>[4x]MVSKGEEDNMASLPATHELHIFGSINGVDFDMVGQGTGNPNEGYEELNLKSTKGDLQFSPWILVPHMGWGFHQYLPYPDGMSPFQAAMVDGSGYQVHRTMQFEDGASLTVNYRYTYEGSHIKGEAQVKGTGFPADGPVMTNSLTAVDSCWSKKTYPNDKTIISTFKWSYTTGNGERYRSTARTTYTFAKPMAANYLKNQPVYVFRKDELKHSETELNFKEWQKAFTDVMGMDELYK

mNeonGreen, an engineered green fluorescent protein (GFP) derived from lancelet, is one of the most brightly fluorescent homologs of Aequorea victoria jellyfish GFP (avGFP) yet reported. However, we were ultimately successful in creating a variant, designated as NeonCyan1, with a tryptophan-derived cyan fluorescent protein (CFP)-type chromophore, and two additional mutants with distinct spectral hues. NeonCyan1 has the ‘double humped’ excitation and emission spectra that are characteristic of FPs with Trp-derived chromophores in the neutral state, such as mTurquoise2 and mCerulean3. To obtain insight into the molecular basis of the empirically determined biophysical and photophysical properties of NeonCyan1 and its variants, we determined the crystal structure of NeonCyan0.95 at close to physiological pH (pH 7.5), NeonCyan0.95 at acidic pH (pH 5.6), and NeonCyan1-T207D at close to physiological pH (pH 6.5).

Screening of a library in which Thr207 was mutated to all other common amino acids led to the identification of two variants with drastically different spectral properties relative to NeonCyan1: Thr207Met (NeonCyan1-T207M) with blue shifted excitation and emission, and Thr207Asp (NeonCyan1-T207D) with red-shifted excitation and emission. To investigate the mechanism of color modifying mutations, we attempted to crystallize the NeonCyan variants under different pH conditions and ultimately obtained the X-ray crystal structure of NeonCyan1-T207D at pH 6.5. This structure revealed that the side chain of the Asp residue at position 207 had displaced the water molecules that had formed a hydrogen bond network from the indole nitrogen to the side chain of Thr207. Accompanying this change was a displacement of the backbone in the vicinity of residue 207 with the Cα of Asp207 in NeonCyan1-T207D positioned 1.2 Å closer to the chromophore than the Cα of Thr207 in NeonCyan0.95. Comparing the structure of NeonCyan0.95 (pH 7.5) with the structure of NeonCyan1-T207D (pH 6.5) revealed that the water-bridged hydrogen bond network that had extended from the indole nitrogen of the chromophore to the hydroxyl of Thr207 was displaced by the side chain of Asp207, and there was a close interaction (2.80 +/− 0.11 Å) between the indole nitrogen and the carboxyl group of Asp207. In contrast to WasCFP and NowGFP, NeonCyan1-T207D has the terminal carboxylate of an aspartate side chain, which typically has a pKa of ~ 4, positioned 2.80 Å from the indole nitrogen. The approximately eight units of mismatch between the pKa of the aspartate side chain and the pKa of the CFP chromophore are incompatible with the co-existence of the anionic chromophore and protonated aspartate. Relative to NeonCyan1, NeonCyan1-T207D has a similar Φ (0.27 versus 0.29) and an increased ε (42 mM−1 cm−1 versus 29 mM−1 cm−1).4-METHOXY-2,3,6-TRIMETHYL-N-(1,3,5-TRIMETHYL-1H-PYRAZOL-4-YL)BENZENESULFONAMIDE | C16 H23 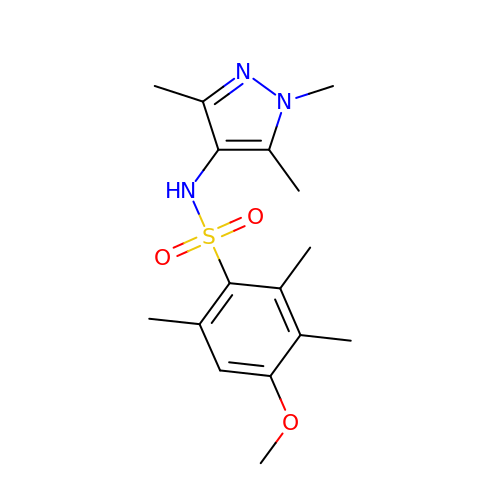N3 O3 S | FHWPTZQYVNRXMX-UHFFFAOYSA-N> MAGIAMKLAKDREAAEGLGSHERAIKYLNQDYETLRNECLEAGALFQDPSFPALPSSLGFKELGPYSSKTRGIEWKRPTEICADPQFIIGGATRTDICQGALGDSWLLAAIASLTLNEEILARVVPLDQSFQENYAGIFHFQFWQYGEWVEVVVDDRLPTKDGELLFVHSAEGSEFWSALLEKAYAKINGCYEALSGGATTEGFEDFTGGIAEWYELRKPPPNLFKIIQKALEKGSLLGCSIDITSAADSEAVTYQKLVKGHAYSVTGAEEVESSGSLQKLIRIRNPWGQVEWTGKWNDNCPSWNTVDPEVRANLTERQEDGEFWMSFSDFLRHYSRLEICNLTPDTLTCDSY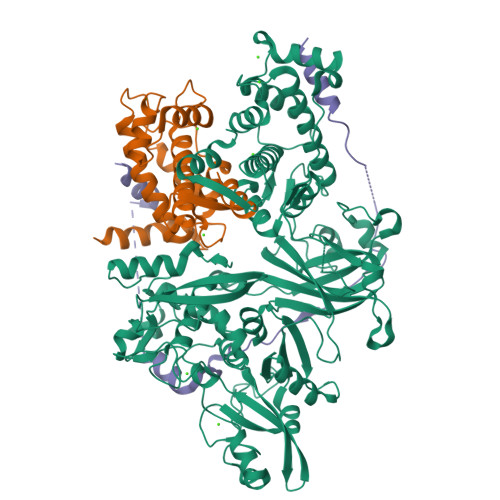KKWKLTKMDGNWRRGSTAGGCRNYPNTFWMNPQYLIKLEEEDEDDEDGERGCTFLVGLIQKHRRRQRKMGEDMHTIGFGIYEVPEELTGQTNIHLSKNFFLTTRARERSDTFINLREVLNRFKLPPGEYVLVPSTFEPHKNGDFCIRVFSEKKADYQTVDDEIEANIEEIEANEEDIGDGFRRLFAQLAGEDAEISAFELQTILRRVLAKREDIKSDGFSIETCKIMVDMLDEDGSGKLGLKEFYILWTKIQKYQKIYREIDVDRSGTMNSYEMRKALEEAGFKLPCQLHQVIVARFADDELIIDFDNFVRCLVRLEILFKIFKQLDPENTGTIQLDLISWLSFSVLGKLAAALEHHHHHH;> MHYSNIEANESEEERQFRKLFVQLAGDDMEVSATELMNILNKVVTRHPDLKTDGFGIDTCRSMVAVMDSDTTGKLGFEEFKYLWNNIKKWQGIYKRFDTDRSGTIGSNELPGAFEAAGFHLNQHIYSMIIRRYSDETGNMDFDNFISCLVRLDAMFRAFRSLDKNGTGQIQVNIQEWLQLTMYS;> MELDDALDELSDSLGQRQPDPDENKPLDDKVKEKIKAEHSEKLGERDDTIPPEYRHLLDNDGKDKPEKPLTKNTEKPGQDQDPIDALSEDLDSCP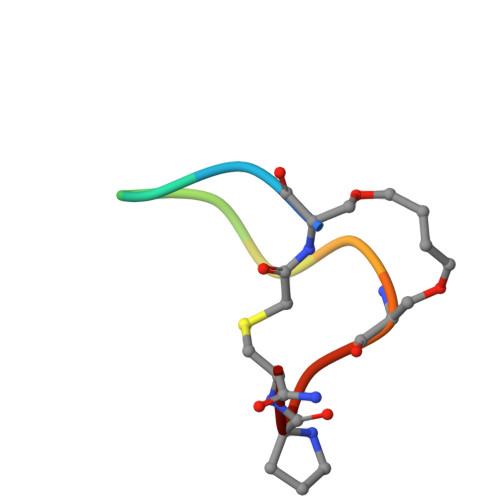> SFEGYDNXFPX5-phenyl-2,4-dihydro-3H-1,2,4-triazol-3-one | C8 H7 N3 O | 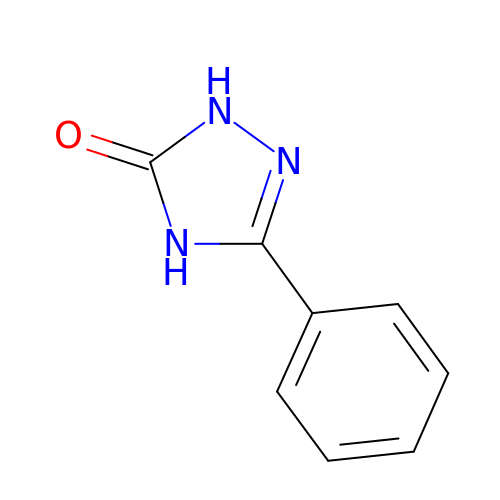FFSXNTGAFSVILG-UHFFFAOYSA-N> PQIINRP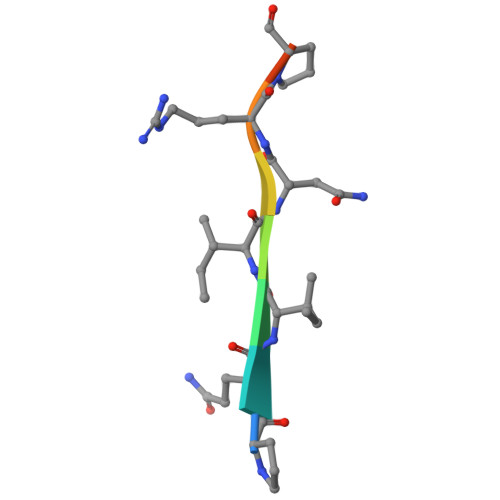QN>MKLLHERMMHSLARYPRQTAVVDEQDALSYEALELRIREFVAMLCALGVGQGQRILLWAHKSVDLVAVMQAALRLGVVYVPVDPLSPVSRLEKIAGDSQAVLVLCTAARLEELAGSALAQVRSVVLDDPASAGYWRNIDTGSSVVPTLAIQPDDLAYILYTSGSTGVPKGVALSHGNALAFVDWACERYCFQPGERFANHAPLHFDLSVLDIYCALNVGATVCLVPESIAFSPRLL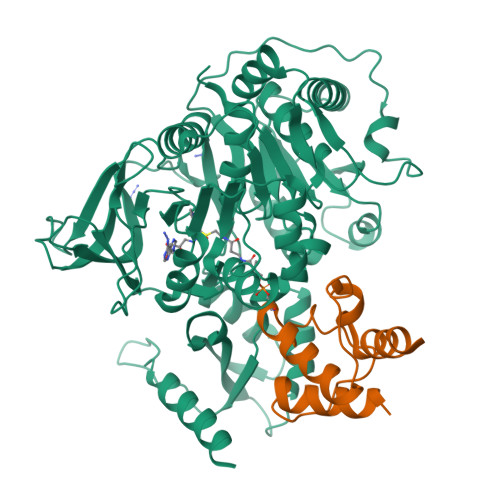TDFIRQHEISIWYSVPSVLMMMMQDGDLLSDIQDTLRVLLFAGEPFPVKHLRDLRAAYADVRLANLFGPTETNVCTAFEVGAIDPERVLPVPIGTAASGNQVWAQKPDGSRCAVGEEGELVVQGPTVMLGYFAKPAQEGPYKTGDMVRQRPDGNYEYLGRRDDMLKVRGNRIERGEVEAALLAHPQVSEAAVLVVGEGMNAQLWGVLVAHTRDALSLIDLKRHCAQRLPRYMIIDKVLCLDALPRNANGKVDRFALARQVEGKLAAALEHHHHHHHH[2x];>[2x]MLESKLINHIATQFLDGEKDGLDSQTPLFELNIVDSAAIFDLVDFLRQESKVSIGMQEIHPANFATVQSMVALVQRLKAHPEQGGAAWEHHHHHH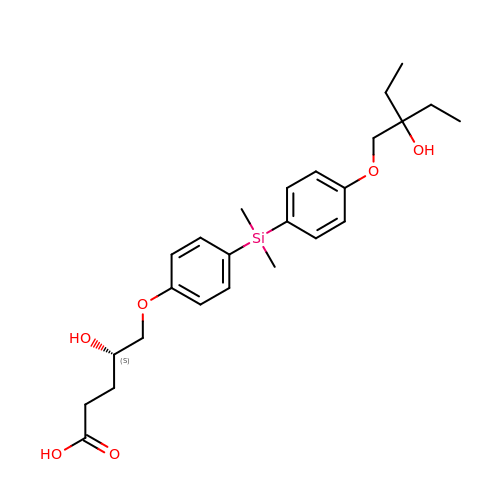(4~{S})-5-[4-[[4-(2-ethyl-2-oxidanyl-butoxy)phenyl]-dimethyl-silyl]phenoxy]-4-oxidanyl-pentanoic acid | C25 H36 O6 Si | OWXFCNNGRPVSBM-LJQANCHMSA-N>MERAEILGVGTELLYGETLDTNTAEIARSLKPYALKVERTLRVADEVAPLAREVEEAFARARLVVLSGGLGPTPDDVTREAVALALGEPLELDEAVLGEIEAFFRARGRAMPEANRKQAMRIPSATWLKNPRGTAPGWWVRKGGKDLVLLPGPPPEWRPMWQEVLPRLGLPRRPYAERVLKTWGIGESEIVERLGPLFVREEEVEVGTYPKVHGVEVVVRGREDRVAELAERIKKKLLKEVWGEGEMTLAEAVKRRMEREGATLSTM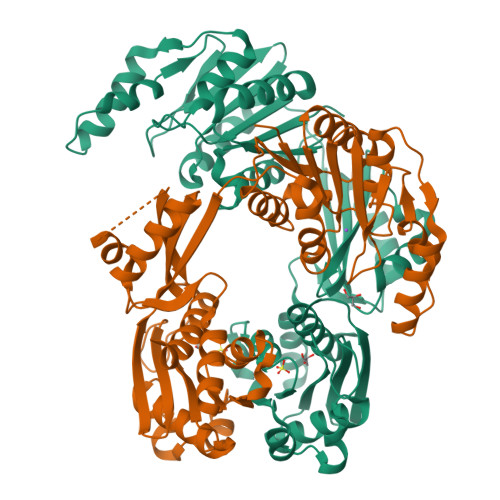ESLTGGLLGAEITRVPGASRFYLGGVVSYSVGAKARFGVPQDLLSRTVSAETARAMAEAARSLFGSTYALATTGVAGPDPLEGEPPGTVYVALAGPTGAEVRRYRFPGDRETVRLRSVYAALALLVT[2x]>[2x]MNKLAVLYAEHIATLQKRTREIIERENLDGVVFHSGQAKRQFLDDMYYPFKVNPQFKAWLPVIDNPHCWIVANGTDKPKLIFYRPVDFWHKVPDEPNEYWADYF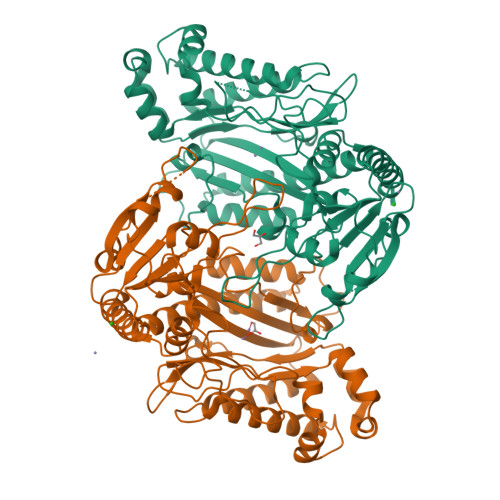DIELLVKPDQVEKLLPYDKARFAYIGEYLEVAQALGFELMNPEPVMNFYHYHRAYKTQYELACMREANKIAVQGHKAARDAFFQGKSEFEIQQAYLLATQHSENDTPFGNYVALNENCAILHYTHFDRVAPATHRSFLIDAGANFNGYAADITRTYDFTGEGEFAELVATMKQHQIALCNQLAPGKLYGELHLDCHQRVAQTLSDFNIVNLSADEIVAKGITSTFFPHGLGHHIGLQLHDVGGFMADEQGAHQEPPEGHPFLRCTRKIEANQVFTIEPGLYFIDSLLGDLAATDNNQHINWDKVAELKPFGGIRIEDNIIVHEDSLENMTRELELD>[2x]GAMEGEEGDDRPREHPFVVTEPGELARGKKNGLDYLFNLYEQAGKFLEEVQHIAREKGEKCPTKVTNQVFRHAKVQGAGYINKPKMR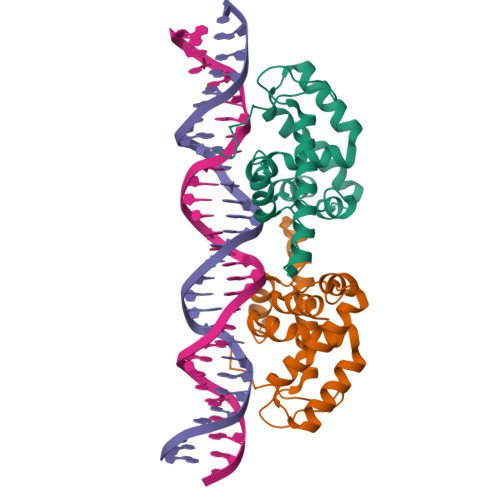QYVHCYALHCLASDKSDELRRCCKERGENVGAWCQACYLPLIKMAKEKSWDIEGLFNSHDKLKIWYVPKKLIQLCHQEKSKH2-[4-(2H-1,4-BENZOTHIAZINE-3-YL)-PIPERAZINE-1-LY]-1,3-THIAZOLE-4-CARBOXYLIC 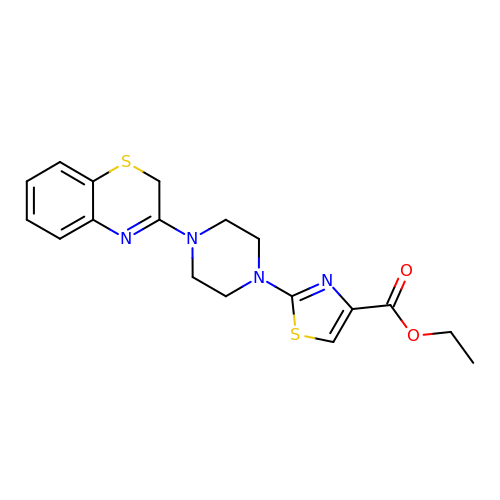ACID ETHYLESTER | C18 H20 N4 O2 S2 | AQJQFCRTSWIUCY-UHFFFAOYSA-N>[4x]MHHHHHAIYNVEVETGDREHAGTDATITIRITGAKGRTDYLKLDKGSFEAGSKEQYTVQGFDVGDIQLIELHSDGGGYWSGDPDWFVNRVIIISSTQDRVYSFPCFRWVIKDMVLFPGEATLPFNEVPAIVSEQRQKELEQRKLTYQWDYVSDDMPGNIKAKTHDDLPRDVQFTDEKSRSYQESRKAALVNLGIGSLFTMFENWDSYDDYHILYRNWILGGTPNMADRWHEDRWFGYQFLNGANPVILTRCDALPSNFPVTNEHVNASLDRGKNLDEEIKDGHIYIVDFKVLVGAKSYGGPVLEDIGYKVPDHLKHDE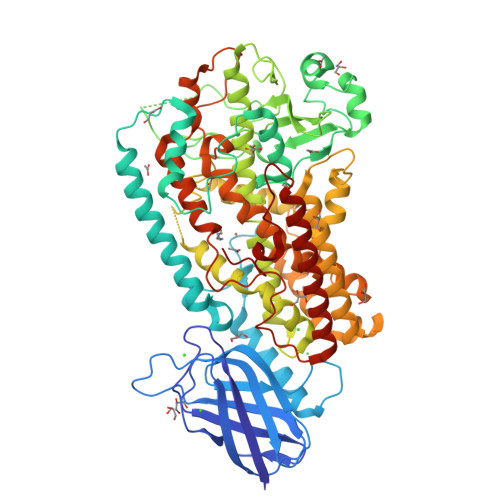ADIRYCAAPLALFYVNKLGHLMPIAIQINQEPGPENPIWTPHEENEHDWMMAKFWLGVAESNFHQLNTHLLRTHLTTESFALSTWRNLASAHPIFKLLQPHIYGVLAIDTIGRKELAGSGGIVDQSLSLGGGGHVTFMEKCFKEVNLQDYHLPNALKKRGVDDPSKLPGFYYRDDGLALWEAIETFIGEIIAIFYKNDDDVKRDNEIQSWIYDVHKNGWRVNPGHQDHGVPASFESREQLKEVLTSLVFTFSCQHAAVNFSQKDHYGFTPNAPAILRHPPPKKKGEATLQSILSTLPSKSQAAKAIATVYILTKFSEDERYLGNYSATAWEDKDALDAINRFQDKLEDISKKIKQRNENLEVPYIYLLPERIPNGTAI>[4x]QVTFAKRRNGLLKKAYELSVLCDAEVALIIFSNRGKLYEFCSSSSMLRTLERYQKCN

The MADS transcription factors (TF) are an ancient eukaryotic protein family. The MIKC domains refer to M, for MADS DBD, I for the dimerisation specifying Intervening domain, K for the coiled-coil keratin-like domain involved in dimer and tetramer formation and C for the variable C-terminal domain important for transactivation and higher-order complex formation. Structural elucidation of the MI domains from the floral regulator, SEPALLATA3 (SEP3), shows a conserved fold with the I domain acting to stabilise the M domain. Taken together, these data demonstrate that the I domain acts as an integral part of the DNA-binding domain and significantly contributes to the functional identity of the MADS TF.

The MADS-box and I domain of SEP3 (SEP3MI, residues 1–90) was used in structural studies as this construct has been shown to be dimeric in solution and to bind DNA in a sequence specific manner. SEP3MI crystallised in space group C2221 with four monomers per asymmetric unit and diffraction to 2.1 Å. The first 18 amino acids, which are predicted to have no defined secondary structure, were disordered as were the 17 C-terminal amino acids, and no electron density was interpretable for these portions of the protein in any of the molecules. Each monomer adopts the same secondary and tertiary structure with an N-terminal alpha helix (α1; aa 18–40) and two antiparallel beta strands (β1; aa 44–48 and β2; aa 55–58). C-terminal to the beta strands is a short loop followed by an alpha helix which is contributed by the I domain (α2; aa 63–73). Each SEP3MI monomer dimerises via extensive contacts between the pairs of alpha helices and beta strands from each partner, with dimerisation required for DNA binding. In the structure, all dimers were formed by crystallographic symmetry, with dimerisation burying over 25% of the total surface area of the molecule. The dimer interface includes hydrophobic interactions between residues in the N-terminal DNA-binding alpha helices, Leu28 and Leu35, and pairs of salt bridges between Glu34 and Arg24. The formation of a four-stranded antiparallel beta sheet further stabilises the quaternary structure of SEP3 with interactions bridging the N-terminal DNA-binding helices and the C-terminal I domain helices. The I domain is anchored to the beta sheet via hydrogen bonding interactions between Glu56 and Tyr70 and pi–cation interactions between Phe48 and Arg69 of the partner monomers.> SMRILLSNDDGVHAPGIQTLAKALREFADVQVVAPDRNRSGASNSLTLESSLRTFTFDNGDIAVQMGTPTDCVYLGVNALMRPRPDIVVSGINAGPNLGDDVIYSGTVAAAMEGRHLGFPALAVSLNGYQHYDTAAAVTCALLRGLSREPLRTGRILNVNVPDLPLAQVKGIRVTRCGSRHPADKVIPQEDPRGNTLYWIGPPGDKYDAGPDTD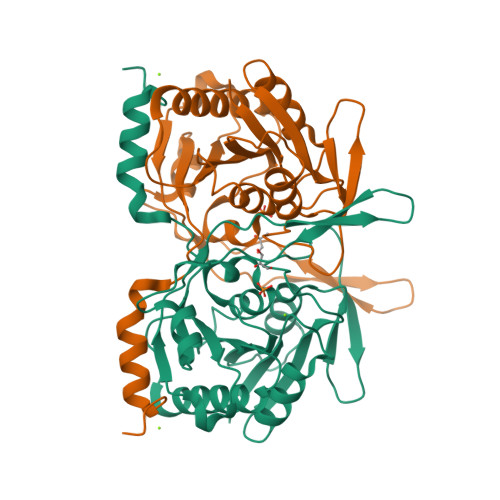FAAVDEGYVSVTPLHVDLTAHSAHDVVSDWLDSVGVGTQW>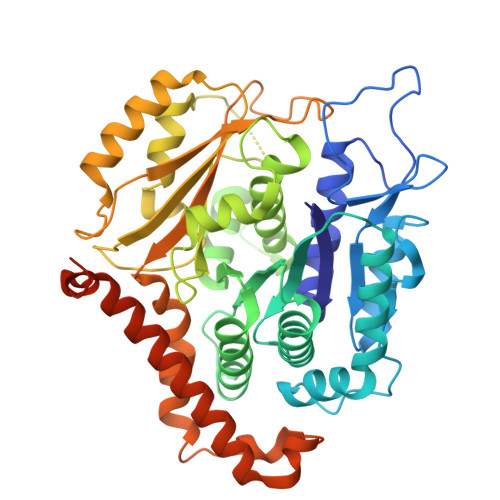 MGGEIITLQAGQCGNHVGKFLWSQLAKEHAIGTDGLSQLPDSSTERDDDTKPFFRENCRNKFTPRAIMMDSEPSVIADVENTFRGFFDPRNTWVASDGASAGNSWANGYDIGTRNQDDILNKIDKEIDSTDNFEGFQLLHSVAGGTGSGLGSNLLEALCDRYPKKILTTYSVFPARSSEVVVQSYNTILALRRLIEDSDATVVFDNASLLNISGKVFRNPNIDLQHTNQLISTIISSVTNSIRFPSYMYSSMSSIYSTLIPSPELHFLSPSFTPFTSDYIHDDIAHKCHSSYDVMLDLLDPSNSLVSTAMNNPTYFNVYNTIIGNVEPRQISRAMTKLQQRIKFPSWSSSAMHVNIGRRSPYLPLQPNENEVSGMMLSNMSTVVNVFENACNTFDKVFAKGAFLNNYNVGDLFQSMQNVQDEFAESREVVQSLMEDYVAAEQDSYLDDVLVDDENMVGELEEDLDADGDHKLV>MGSSHHHHHHSQDPMSLNLVSEQLLAANGLKHQDLFAILGQLAERRLDYGDLYFQSSYHESWVLEDRIIKDGSYNIDQGVGVRAISGEKTGFAYADQISLLALEQSAQAARTIVRDSGDGKVQTLGAVEHSPLYTSVDPLQSMSREEKLDILRRVDKVAREADKRVQEVTASLSGVYELILVAATDGTLAADVRPLVRLSVSVLVEEDGKRERGASGGGGRFGYEFFLADLDGEVRADAWAKEAVRMALVNLSAVAAPAGTMPVVLGAGWPGVLLHAAVGHGLEGDFNRRGTSVFSGQVGELVASELCTVVDDGTMVDRRGSVAIDDEGTPGQYNVLIENGILKGYMQDKLNARLMGMTPTGNGRRESYAHLPMPRMTNTYMLPGKSTPQEIIESVEYGIYAPNFGGGQVDITSDKFVFSTSEAYLIENGKVTKPVKGATLIGSGIETMQQISMVGNDLKLDNGVGVCGKEGQSLPVGVGQPTLKVDNLTVGGTA[2x];>MALAMKVISQVEAQRKILEEAVSTALELASGKSDGAEVAVSKTTGISVSTRYGEVENVEFNSDGALGITVYHQNRKGSASSTDLSPQAIARTVQAALDIARYTSPDPCAGVADKELLAFDAPDLDLFHPAEVSPDEAIELAARAEQAALQADKRITNTEGGSFNSHYGVKVFGNSHGMLQGYCSTRHSLSSCVIAEENGDMERDYAYTIGRAMSDLQTPEWVGADCARRTLSRLSPRKLSTMKAPVIFANEVATGLFGHLVGAIAGGSVYRKSTFLLDSLGKQILPDWLTIEEHPHLLKGLASTPFDSEGVRTERRDIIKDGILTQWLLTSYSARKLGLKSTGHAGGIHNWRIAGQGLSFEQMLKEMGTGLVVTELMGQGVSAITGDYSRGAAGFWVENGEIQYPVSEITIAGNLKDMWRNIVTVGNDIETRSNIQCGSVLLPEMKIAGQ[2x];>VLEDRI[2x]

Using a combination of biochemical and crystallographic methods we show that E. coli TldD and TldE interact to form a heterodimeric metalloprotease. TldD/E cleaves the N-terminal leader sequence from the modified MccB17 precursor peptide, to yield mature antibiotic, while it has no effect on the unmodified peptide. Both proteins are essential for the activity; however, only the TldD subunit forms a novel metal-containing active site within the hollow core of the heterodimer. Peptide substrates are bound in a sequence-independent manner through β sheet interactions with TldD and are likely cleaved via a thermolysin-type mechanism.

Attempts were made to trap uncleaved peptides in the active site of TldD through the use of a catalytically inactive Glu263Ala mutant. Surprisingly, the resultant density was essentially the same in every case, irrespective of the added ligand. We therefore focused on the highest resolution dataset, which had been collected to 1.45-Å resolution after co-crystallization with the engineered angiotensin variant described above. Clear density was present for the backbone of a hexapeptide spanning subsites S3-S3’ (hence E263A-hex) and, for four of the residues, probable identities could be assigned based on side-chain density to give an x-Leu-x-Asp-Arg-Ile sequence. This bore no resemblance to any of the added ligands, but curiously gave a match with residues 49–54 of TldD itself. A possible explanation for this could be that proteolytic fragments of the overexpressed TldD protein are comparatively abundant in the expression host, and this particular fragment binds with high affinity, principally due to the Asp residue in subsite S1′, the side chain of which does not occupy the pocket used by the n-pentyl chain of actinonin, but rather chelates the catalytic zinc. Remarkably, hydrogen bonding is restricted to backbone atoms only, such that the peptide acts as an additional β strand that effectively fuses the β sheet and the β barrel motifs in the C-terminal domain of TldD through anti-parallel interactions with both supersecondary structural elements that extend from subsite S2 to S2′ inclusive. Furthermore, binding of the hexapeptide does not result in any significant conformational changes. When compared against the phosphate-bound structure, the RMSD after superposing TldD Cα atoms was only 0.33 Å (averaged across both copies of the subunit in the asymmetric unit).> EE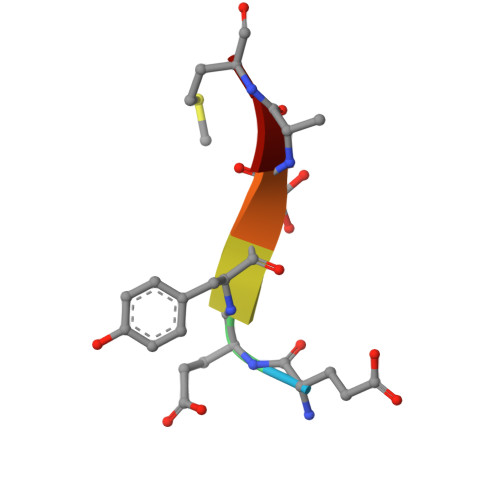YSAM>HRILIERQEKSDTNFKEFVIKKLQKNCQCSPAKAKNMILGFLPVLQWLPKYDLKKNILGDVMSGLIVGILLVPQSIAYSLLAGQEPVYGLYTSFFASIIYFLLGTSRHISVGIFGVLCLMIGETVDRELQKAGYDNAHSAPSLGMV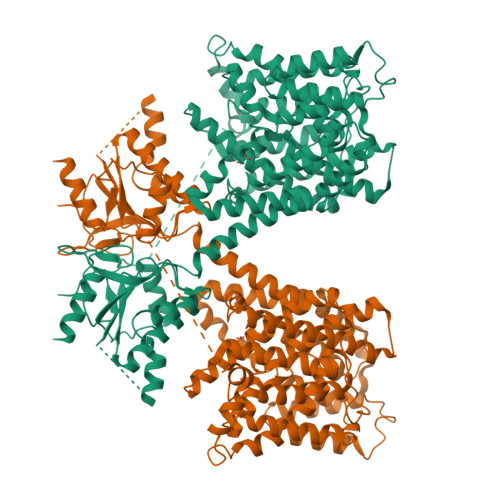SNGSTLLNHTSDRICDKSCYAIMVGSTVTFIAGVYQVAMGFFQVGFVSVYLSDALLSGFVTGASFTILTSQAKYLLGLNLPRTNGVGSLITTWIHVFRNIHKTNLCDLITSLLCLLVLLPTKELNEHFKSKLKAPIPIELVVVVAATLASHFGKLHENYNSSIAGHIPTGFMPPKVPEWNLIPSVAVDAIAISIIGFAITVSLSEMFAKKHGYTVKANQEMYAIGFCNIIPSFFHCFTTSAALAKTLVKESTGCHTQLSGVVTALVLLLVLLVIAPLFYSLQKSVLGVITIVNLRGALRKFRDLPKMWSISRMDTVIWFVTMLSSALLSTEIGLLVGVCFSIFCVILRTQKPKSSLLGLVEESEVFESVSAYKNLQIKPGIKIFRFVAPLYYINKECFKSALYKQTVNPILIKVAWKKAAKRKIKEKVVTLGGIQDEMSVQLSHDPLELHTIVIDCSAIQFLDTAGIHTLKEVRRDYEAIGIQVLLAQCNPTVRDSLTNGEYCKKEEENLLFYSVYEAMAFAEVSKN[2x]Here we describe efficient routes starting from validated parallel and antiparallel peptide assemblies to design two families of α-helical barrel proteins with central channels that bind small molecules. Computational designs are seeded by the sequences and structures of defined de novo oligomeric barrel-forming peptides, and adjacent helices are connected by loop building. For targets with antiparallel helices, short loops are sufficient. However, targets with parallel helices require longer connectors; namely, an outer layer of helix–turn–helix–turn–helix motifs that are packed onto the barrels.

The parallel α-helical barrel proteins required a different design approach, as sequence-to-structure relationships for the g-a-d-e positions were available to seed the designs, but connecting adjacent parallel helices was not straightforward because of the need to span ~40 Å along the structures. We exploited the Cn symmetry of the parallel α-helical barrel peptides to generate helix–turn–helix–turn–helix units, which could be repeated about the Cn axis to close structures with n central helices and n−1 buttressing helices. Encouraged by the successful design of sc-apCC-6 and sc-CC-7, we extended the seeded design approaches to target α-helical barrel proteins with five, six and eight central helices. By contrast, the six- and eight-helix-based targets bound dye, consistent with accessible cavities, which were confirmed by SEC-SAXS and X-ray crystal structures solved using molecular replacement. Together, these additional designs delivered the de novo proteins sc-CC-5, sc-CC-6 and sc-CC-8. For the parallel targets, the experimental structures show minor fraying at the C termini of the inner helices compared with the seeds and models, which appears to improve the packing of the external three-helix bundles. However, the symmetry of the central parallel helices is maintained. The backbone RMSD values for the repeating helix–turn–helix–turn–helix motifs are ≤0.5 Å, which is expected given the low sequence variation in the loops and the hydrophobic cores of these buttressing helices. The parallel designs all showed some similarity with natural and designed helical solenoid proteins. This was anticipated because the helix–turn–helix–turn–helix tertiary fragments used as connectors came from a set of de novo proteins of this type64.

>[2x]GSHMGIAEALKLIAEALEVIAKALLAIALGDKELAKEALKEAEEVKKKAEKLKKEAEKKGDRIAAALALIAIALAVIALALVAIALGDKELAKKAKEEALKVLKEAEKGYKEAKKQGDEIAAALYLIAIALAAIALALVAIALGDEELAKKAKELAEKVKEEAEKRYKEAEKQGDEIAKALYLIAIALAAIALALVAIALKDEKLAKEALKLALEVKKKSEEEYEEAKKQGNEIAKALYLIAIALAAIALALVAIALKDEELAEEAKEEAEKVKEEAEKQAKEAKEQGNEIAKSLYKIAISLAEIALSLAEIAKS2-acetamido-2-deoxy-beta-D-allopyranose | C8 H15 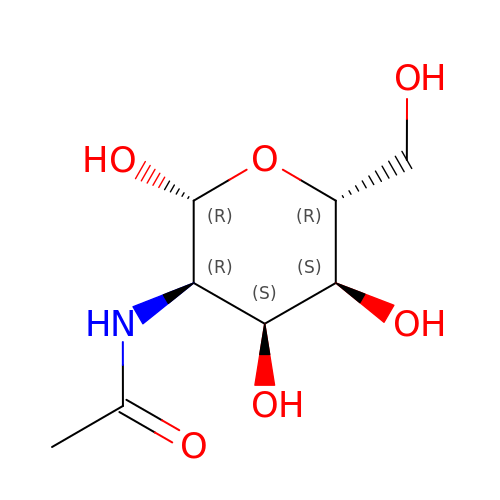N O6 | OVRNDRQMDRJTHS-UIAUGNHASA-N S-HEXYLGLUTATHIONE | C16 H30 N3 O6 S | 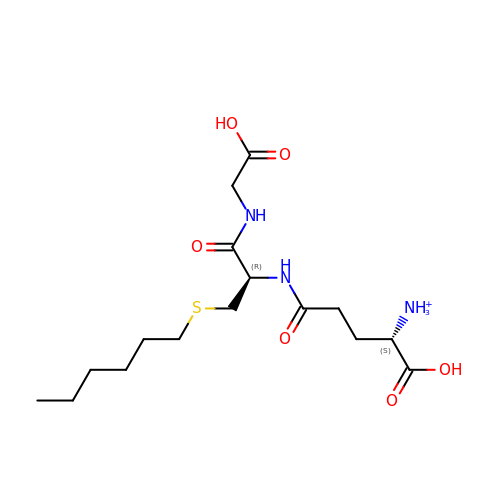HXJDWCWJDCOHDG-RYUDHWBXSA-O>[4x]MTDSSSLRGVDADTEKRINVGKKHLQTLRNLETRCHDSLQALVVIDAGSSSTRTNVFLAKTRSCPNKGRSIDPDSIQLIGAGKRFAGLRVVLEEWLDTYAGKDWESRPVDARLLFQYVPQMHEGAKKLMQLLEEDTVAILDSQLNEKQKVQVKALGIPVMLCSTAGVRDFHEWYRDALFVLLRHLINNPSPAHGYKFFTNPFWTRPITGAEEGLFAFITLNHLSRRLGEDPARCMIDEYGVKQCRNDLAGVVEVGGASAQIVFPLQEGTVLPSSVRAVNLQRERLLPERYPSADVVSVSFMQLGMASSAGLFLKELCSNDEFLQGGICSNPCLFKGFQQSCSAGEVEVRPDGSASVNEDVRKNRLKPLATYCSVNNPEISFKVTNEMQCRENSIDPT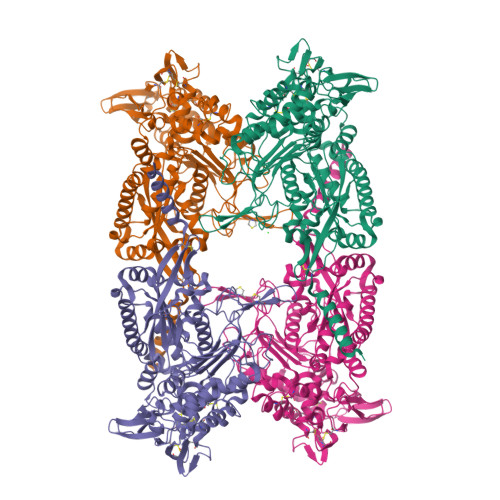KPLAERMKIENCSIIKGTGNFDKCVSQVESILVAPKLPLPANIEAASSGFESVDQVFRFASSTAPMIVTGGGMLAAINTLKDHRLLRSDFSGDVEELAEAAREFCSSEVIIRTDGPVIQLPNARGEQKLNSLNFDLCKTMALTVSLLRHMAAGENQPSFIKWEKSIAGPDGKPLADLGWQVGVILHHVLFTEEWGRNAYEAGYSHNLEHHHHHH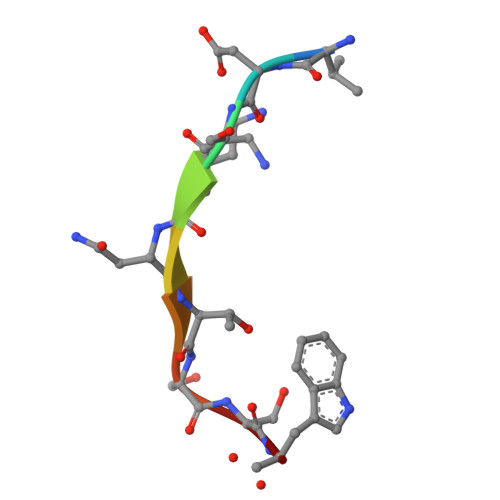> VDSKNTSSW>GPHMMIDLRSDTVTKPTEEMRKAMAQAEVGDDVYGEDPTINELERLAAETFGKEAALFVPSGTMGNQVSIMAHTQRGDEVILEADSHIFWYEVGAMAVLSGVMPHPVPGKNGAMDPDDVRKAIRPRNIHFPRTSLIAIENTHNRSGGRVVPLENIKEICTIAKEHGINVHIDGARIFNASIASGVPVKEYAGYADSVMFCLSKGLCAPVGSVVVGDRDFIERARKARKMLGGGMRQAGVLAAAGIIALTKMVDRLKEDHENARFLALKLKEIGYSVNPEDVKTNMVILRTDNLKVNAHGFIEALRNSGVLANAVSDTEIRLVTHKDVSR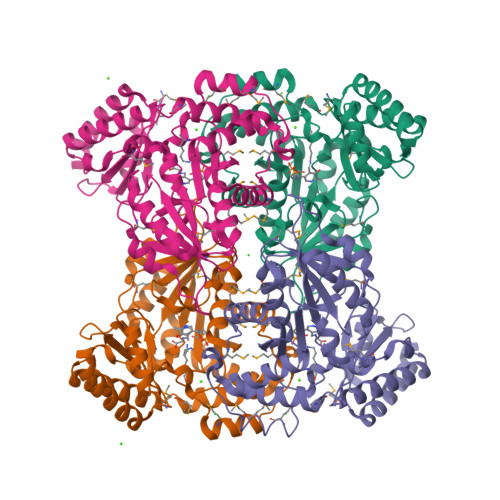NDIEEALNIFEKLFRKFS[4x]>[2x]SQGRACLSKAELTADLIWLSANRTGEESAEELNYSGCDLSGLSLVGLNLSSVNFSGAVLDDTDLRMSDLSQAVLENCSFKNSILNECNFCYANLSNCIIRALFENSNFSNSNLKNASFKGSSYIQYPPILNEADLTGAIIIPGMVLSGAILGDVKELFSEKSNTI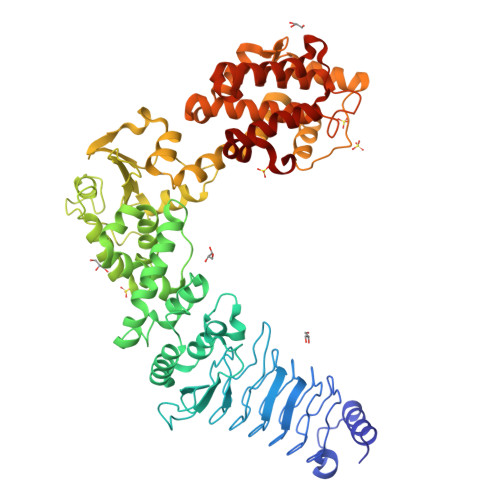NLGGCYIDLSDIQENILSVLDNYTKSNKSILLTMNTSDDKYNHDKVRAAEELIKKISLDELAAFRPYVKMSLADSFSIHPYLNNANIQQWLEPICDDFFDTIMSWFNNSIMMYMENGSLLQAGMYFERHPGAMVSYNSSFIQIVMNGSRRDGMQERFRELYEVYLKNEKVYPVTQQSDFGLCDGSGKPDWDDDSDLAYNWVLLSSQDDGMAMMCSLSHMVDMLSPNTSTNWMSFFLYKDGEVQNTFGYSLSNLFSESFPIFSIPYHKAFSQNFVSGILDILISDNELKERFIEALNSNKSDYKMIADDQQRKLACVWNPFLDGWELNAQHVDMIMGSHVLKDMPLRKQAEILFCLGGVFCKYSSSDMFGTEYDSPEILRRYANGLIEQAYKTDPQVFGSVYYYNDILDRLQGRNNVFTCTAVLTDMLTEHAKESFPEIFSLYYPVAWR>MSVVTTRARIAETLTEKHTLGIEKVVATD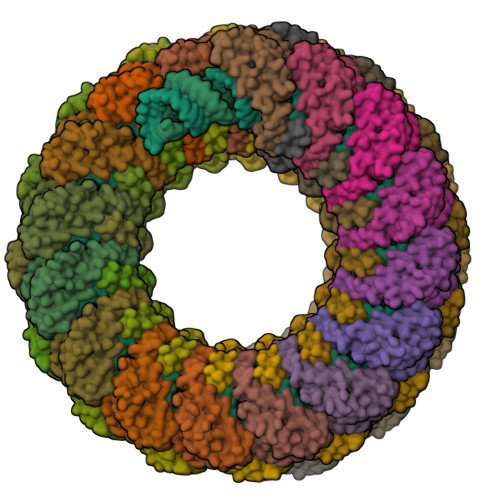SWRVGITSREKKLERINISAEISRRIQDEAIAYARNKGIPYLPGINGIAWKLLRLKWLGYTDQINVVMRTVPAEWRDFLTQIMENTQMESMYSELRKVRV[23x];>[23x]MSVEVYRQKIEKGGYSAAYEATRRYEREEIEVLSWSSRWESAWSKFGEAVKALGKIEGAPRALVIAKVQEALAYMSKPLPNMKLAMAAAVQAVRACEQLPGMNRERCLDAVAGALGVAKDWIRREMTGGGGGGGGGGGGGGGAVV> SFVDHPPDWLEEVGEGLREFLGLEAGPPKPKPNQQHQDQARGLVLPGYNYLGPGNGLDRGEPVNRADEVAREHDISYNEQLEAGDNPYLKYNHADAEFQEKLADDTSFGGNLGKAVFQAKKRVLEPFGLVEEGAKTAPTGKRIDDHFPKRKKARTEEDSKPSTSSDAEAGPSGSQQLQIPA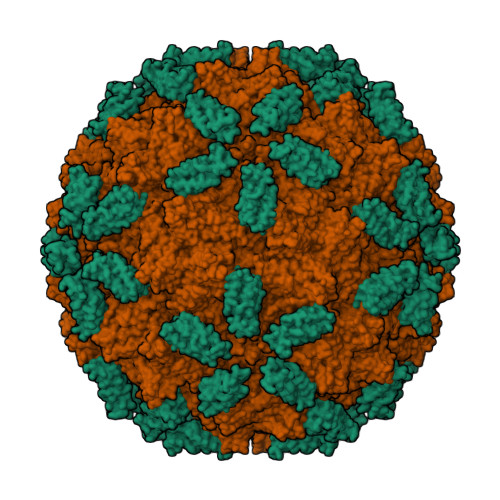QPASSLGADTMSAGGGGPLGDNNQGADGVGNASGDWHCDSTWMGDRVVTKSTRTWVLPSYNNHQYREIKSGSVDGSNANAYFGYSTPWGYFDFNRFHSHWSPRDWQRLINNYWGFRPRSLRVKIFNIQVKEVTVQDSTTTIANNLTSTVQVFTDDDYQLPYVVGNGTEGCLPAFPPQVFTLPQYGYATLNRDNTENPTERSSFFCLEYFPSKMLRTGNNFEFTYNFEEVPFHSSFAPSQNLFKLANPLVDQYLYRFVSTNNTGGVQFNKNLAGRYANTYKNWFPGPMGRTQGWNLGSGVNRASVSAFATTNRMELEGASYQVPPQPNGMTNNLQGSNTYALENTMIFNSQPANPGTTATYLEGNMLITSESETQPVNRVAYNVGGQMATNNQSSTTAPATGTYNLQEIVPGSVWMERDVYLQGPIWAKIPETGAHFHPSPAMGGFGLKHPPPMMLIKNTPVPGNITSFSDVPVSSFITQYSTGQVTVEMEWELKKENSKRWNPEIQYTNNYNDPQFVDFAPDSTGEYRTTRPIGTRYLTRPL;> MASHHHHHHVSAGESVQITLPKNEVQLNAYVLQEPPKGETYTYDWQLITHPRDYSGEMEGKHSQILKLSKLTPGLYEFKVIVEGQNAHGEGYVNVTVKPEPRKNRPPIAIVSPQFQEISLPTTSTVIDGSQSTDDDKIVQYHWEELKGPLREEKISEDTAILKLSKLVPGNYTFSLTVVDSDGATNSTTANLTVNKAVD>GSDSGTEEYELNGGLPPGTPGSPDASPARWGWRHGPINVNHYASKKSAAESMLDIALLMANASQLKAVVEQGPSFAFYVPLVVLISISLVLQIGVGVLLIFLVKYDLNNPAKHAKLDFLNNLATGLVFIIVVVNIFITAFGVQK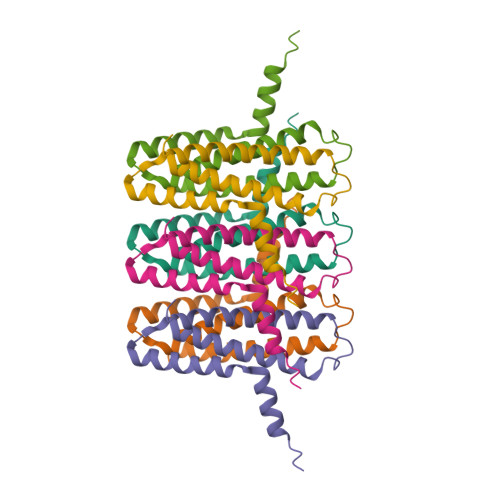PLMDMAPQQ[6x]>[4x]GSALPILLDCDPGHDDAIAIVLALASPELDVKAITSSAGNQTPEKTLRNVLRMLTLLNRTDIPVAGGAVKPLMRELIIADNVHGESGLDGPALPEPTFAPQNCTAVELMAKTLRESAEPVTIVSTGPQTNVALLLNSHPELHSKIARIVIMGGAMGLGNWTPAAEFNIYVDPEAAEIVFQSGIPVVMAGLDVTHKAQIHVEDTERFRAIGNPVSTIVAELLDFFLEYHKDEKWGFVGAPLHDPCTIAWLLKPELFTSVERWVGVETQGKYTQGMTVVDYYYLTGNKPNATVMVDVDRQGFVDLLADRLKFYA

Pyrimidine-preferring nucleoside hydrolases (CU-NHs) are members of the broad family of Ca2+-dependent hydrolases that catalyze the cleavage of the N-glycosidic bond in nucleosides. Two CU-NH-encoding genes are present in E. coli cells, termed either ybeK and yeiK, or rihA and rihB, respectively. The gene products RihA and RihB have been characterized using steady-state kinetics and X-ray crystallography, and display similar kinetic constants, characterized by mid- to high-micromolar KM values for uridine and cytidine. The structure of each monomer maintains the α/β fold that is typical of NHs, with the Ca2+-containing active site located in a deep, narrow cavity at the C-terminal end of a core 10-stranded β-sheet surrounded by α-helices.

Here, we report the crystal structure of the complex between the E. coli RihA enzyme and the competitive inhibitor 3,4-diamino phenyliminoribitol (DAPIR) to a resolution of 2.1 Å. The molecular replacement method unambiguously identified four independent molecules in the asymmetric unit, arranged as a tetramer with the subunits related by 222 symmetry. The DAPIR molecule is bound at the RihA active site in two conformations, differing in the orientation of the diaminophenyl group. The N3 amino group of DAPIR can either be directed towards the α9 helix of RihA (as found in chain A, as per PDB file nomenclature), or towards the αL loop (chains B and D). In agreement with the mode of binding of ribonucleoside analogues to group I NHs observed by X-ray crystallography, the binding between DAPIR and the calcium metal centre in RihA occurs through the 2' and 3'-hydroxyl groups of the ribose moiety, and is further strengthened by hydrogen bonding of the hydroxyl group in O5' to Asn158 and Glu164. The octacoordination of the calcium ion involves the DAPIR 2' and 3'-hydroxyls, the carboxylates of three Asp residues at positions 10, 15, and 241, the Thr124 backbone oxygen, and a water molecule. The diaminophenyl ring of the inhibitor, mimicking the nitrogenous base of substrates, establishes only van der Waals' interactions with the side chains of Ala78, Val81, Phe165, Phe223, and Lys228. In this polypeptide chain, residues Asn80-Val81-His82-Gly83 assume a helical conformation (αL), allowing the side chains of residues Val81 and His82 to face the inner portion of the active site and interact with the aromatic ring of DAPIR. In the closed structure, the highly conserved His82 residue of the αL loop is interacting via a hydrogen bond between its Nδ side chain atom and the corresponding atom of His13, in a side-by-side orientation. The structure of RihA with the inhibitor DAPIR describes the enzyme structural rearrangement and interactions when bound to an active site ligand, underscores a buttressing role of the tetrameric assembly, and provides a snapshot of a structure sampled along the reaction coordinate.> MAEQSDKAVK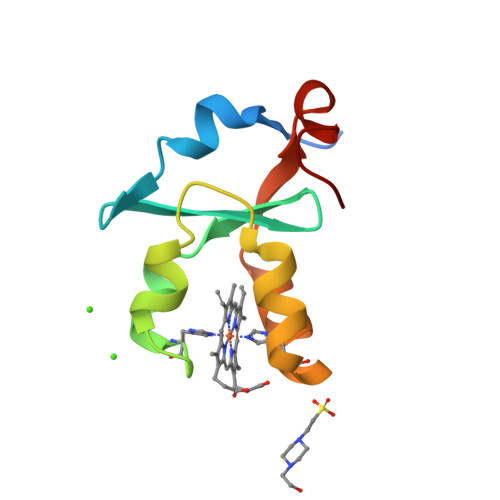YYTLEEIQKHNNSKSTWLILHHKVYDLTKFLEEHPGGEEVLREQAGGDATENFEDVGHSTDARELSKTFIIGELHPDDRSKIAK> SEFTTDPVRMYMREMGTVELLTREGEIDIAKRIEDGINQVQCSVAEYPEAITYLLEQYDRVEAEEARLSDLITGFVDPNAEEDLAPTATHVGSELSQEDLDDDEDEDEEDGDDDSADDDNSIDPELAREKFAELRAQYVVTRDTIKAKGRSHATAQEEILKLSEVFKQFRLVPKQFDYLVNSMRVMMDRVRTQERLIMKLCVEQCKMPKKNFITLFTGNETSDTWFNAAIAMNKPWSEKLHDVSEEVHRALQKLQQIEEETGLTIEQVKDINRRMSIGEAKARRAKKEMVEANLRLVISIAKKYTNRGLQFLDLIQEGNIGLMKAVDKFEYRRGYKFSTYATWWIRQAITRSIADQARTIRIPVHMIETINKLNRISRQMLQEMGREPTPEELAERMLMPEDKIRKVLKIAKEPISMETPIGDDEDSHLGDFIEDTTLELPLDSATTESLRAATHDVLAGLTAREAKVLRMRFGIDMNTDYTLEEVGKQFDVTRERIRQIE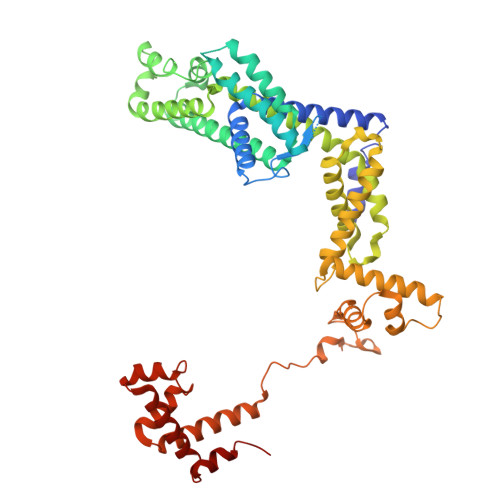AKALRKLRHPSRSEVLRSFLDD>GPHMTVLSDSAHFDVKHPLNTAWTLWYTKPAVDKSESWSDLLRPVTSFQTVEEFWAIIQNI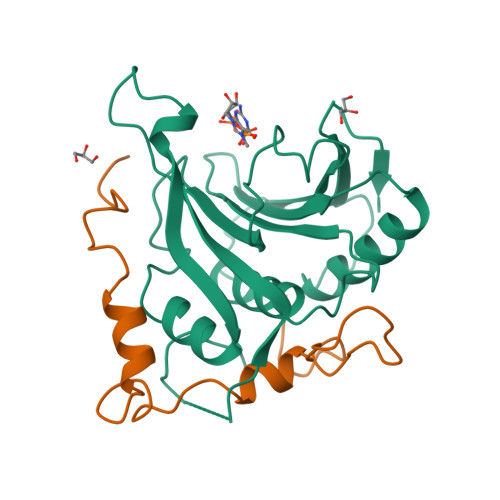PEPHELPLKSDYHVFRNDVRPEWEDEANAKGGKWSFQLRGAGADIDELWLRTLLAVIGETIDEDDSQINGVVLSIRKGGNKFALWTASEDKEPLLRIGGKFKQVLALTDDGHLEFFPHSSANGRHPQPSITL[2x];>GPHMTDPITNYKPMDLQYKTYAYSMNELYHLKPSLASASYEEDPLISELVRSLPKRKFWRLRMG[2x]>[4x]FTREDYVFMAQLNENAERYDEMVETMRKISGMEGELSDKERNLLSVAYKNVIGPR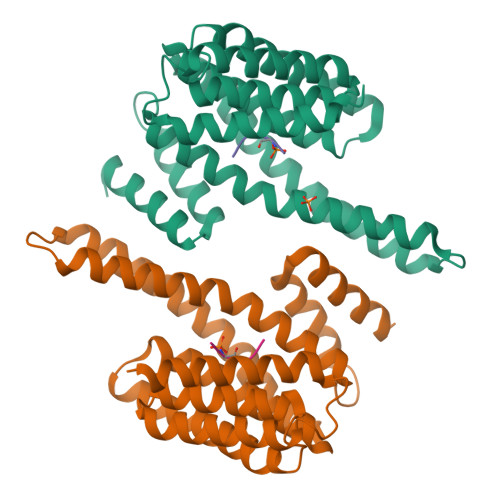RAAWRIVSSIEAKEKGRQKPNAKRIEQIRVYRQKIEKELSDICNDILKLLQEQFVPRSTNADAKVFYYKMQGDYYRYLAEYSSGEDKEKIAGSALNAYNSAFEISQQLPPTHPIRLGLALNFSVFYYEILASPDRACELARKAFDAAITDLDKLTEESYKDSTLIMQLLRDNLNLWVTD;>[4x]ARAASAPA>[2x]MGSSHHHHHHENLYFQGEKIQSTKVDKVPTLKAERLAMINITAGANSATTQAANTRQERTPKLEKAPNTNEEKTSASKIEKISQPKQEEQKTLNISATPAPKQEQSQTTTESTTPKTKVTTPP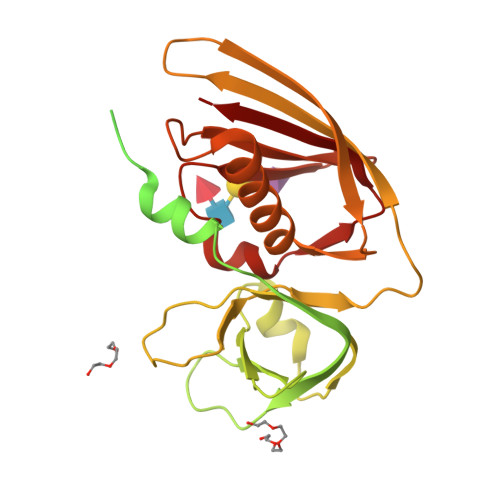STNTPQPMQSTKSDTPQSPTIKQAQTDMTPKYEDLRAYYTKPSFEFEKQFGFMLKPWTTVRFMNVIPNRFIYKIALVGKDEKKYKDGPYDNIDVFIVLEDNKYQLKKYSVGGITKTNSKKVNHKVELSITKKDNQGMISRDVSEYMITKEEISLKELDFKLRKQLIEKHNLYGNMGSGTIVIKMKNGGKYTFELHKKLQEHRMADVIDGTNIDNIEVNIK>MTMSLEVFEKLEAKVQ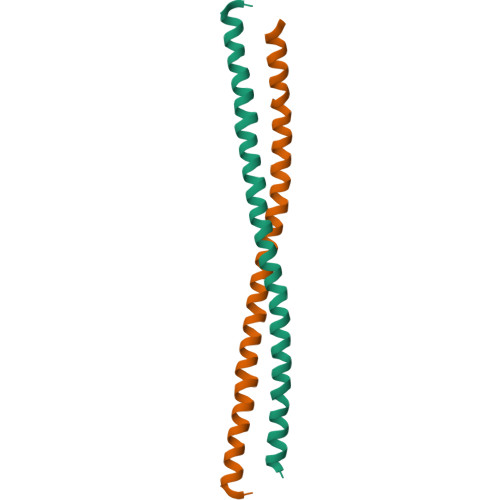QAIDTITLLQMEIEELKEKNNSLSQEVQNAQHQREELERENNHLKEQQNGWQERLQALLGRMEEV[4x]>GMSDFDLIVVGSGLFGLTVAERAASQLGKKVLIVEKRSHLGGNAYSEAEPETGIEIHKYGAHLFHTSNKRVWDYVNQFTAFTGYQHRVFAMHNGTAYQFPMGLGLINQFFGRYYTPDEARELIKEQSAEIDSKDATNLEEKAISLIGRPLYEAFIRDYTAKQWQTDPKELPAGNITRLPVRYNFDNRYFNDTYEGLPVDGYAQWLSNMADHENIEVRLDTDWFEVREDLRAQNPEAPVVYTGPLDRYFDYSEGHLGWRTLDFETEVLNTGDFQGTPVMNYNDAEFPYTRIHEFRHFHPEREDRHPKDKTVIMKEYSRFAEEGDEPYYPINTPSDREMLFKYRELADAETESGKVYFGGRLGTYQYLDMHMAIASALSMFDNKLVDA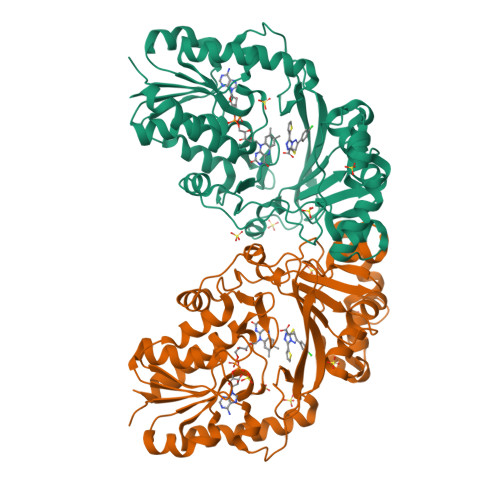LK[2x]> DYKDDDDKSHSPHLPRPHSRVPPHPSSERRAVYIGALFPMSGGWPGGQACQPAVEMALEDVNSRRDILPDYELKLIHHDSKCDPGQATKYLYELLYNDPIKIILMPGCSSVSTLVAEAARMWNLIVLSYGSSSPALSNRQRFPTFFRTHPSATLHNPTRVKLFEKWGWKKIATIQQTTEVFTSTLDDLEERVKEAGIEITFRQSFFSDPAVPVKNLKRQDARIIVGLFYETEARKVFCEVYKERLFGKKYVWFLIGWYADNWFKIYDPSINCTVDEMTEAVEGHITTEIVMLNPANTRSISNMTSQEFVEKLTKRLKRHPEETGGFQEAPLAYDAIWALALALNKTSGGGGRSGVRLEDFNYNNQTITDQIYRAMNSSSFEGVSGHVVFDASGSRMAWTLIEQLQGGSYKKIGYYDSTKDDLSWSKTDKWIGGSPPADQTLVIKTFRFLSQKLFISVSVLSSLGIVLAVVCLSFNIYNSHVRYIQNSQPNLNNLTAVGCSLALAAVFPLGLDGYHIGRNQFPFVCQARLWLLGLGFSLGYGSMFTKIWWVHTVFTKKEEKKEWRKTLEPWKLYATVGLLVGMDVLTLAIWQIVDPLHRTIETFAKEEPKEDIDVSILPQLEHCSSRKMNTWLGIFYGYKGLLLLLGIFLAYETKSVSTEKINDHRAVGMAIYNVAVLCLITAPVTMILSSQQDAAFAFASLAIVFSSYITLVVLFVPKMRRLITRGEWQSEAQDTMKTGSSTNNNEEEKSRLLEKENRELEKIIAEKEERVSELRHQLQSRQQLRSRRHPPTPPEPSGGLPRGPPEPPDRLSCDGSRVHLLYKHHHHHH;> DYKDDDDKWARGAPRPPPSSPPLSIMGLMPLTKEVAKGSIGRGVLPAVELAIEQIRNESLLRPYFLDLRLYDTECDNAKGLKAFYDAIKYGPNHLMVFGGVCPSVTSIIAESLQGWNLVQLSFAATTPVLADKKKYPYFFRTVPSDNAVNPAILKLLKHYQWKRVGTLTQDVQRFSEVRNDLTGVLYGEDIEISDTESFSNDPCTSVKKLKGNDVRIILGQFDQNMAAKVFCCAYEENMYGSKYQWIIPGWYEPSWWEQVHTEANSSRCLRKNLLAAMEGYIGVDFEPLSSKQIKTISGKTPQQYEREYNNK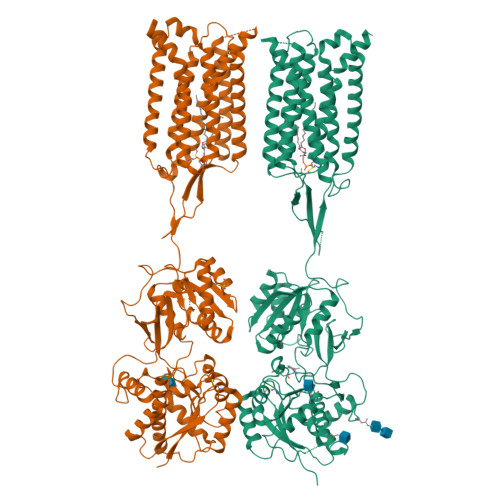RSGVGPSKFHGYAYDGIWVIAKTLQRAMETLHASSRHQRIQDFNYTDHTLGRIILNAMNETNFFGVTGQVVFRNGERMGTIKFTQFQDSREVKVGEYNAVADTLEIINDTIRFQGSEPPKDKTIILEQLRKISLPLYSILSALTILGMIMASAFLFFNIKNRNQKLIKMSSPYMNNLIILGGMLSYASIFLFGLDGSFVSEKTFETLCTVRTWILTVGYTTAFGAMFAKTWRVHAIFKNVKMKKKIIKDQKLLVIVGGMLLIDLCILICWQAVDPLRRTVEKYSMEPDPAGRDISIRPLLEHCENTHMTIWLGIVYAYKGLLMLFGCFLAWETRNVSIPALNDSKYIGMSVYNVGIMCIIGAAVSFLTRDQPNVQFCIVALVIIFCSTITLCLVFVPKLITLRTNPDAATQNRRFQFTQNQKKEDSKTSTSVTSVNQASTSRLEGLQSENHRLRMKITELDKDLEEVTMQLQDTPEKTTYIKQNHYQELNDILNLGNFTESTDGGKAILKNHLDQNPQLQWNTTEPSRTCKDPIEDINSPEHIQRRLSLQLPILHHAYLPSIGGVDASCVSPCVSPTASPRHRHVPPSFRVMVSGL>METRDDFMFELSDKPLLPCYNLQVSVSRGPCNWFLFSDVLKRLKLSSRIFQARFPHFEITTMPKAEFYRQVASSQLLTPAERPGGLDDRSPPGSSETVELVRYEPDLLRLLGSEVEFQSCNS[2x];>QGTREQLNLCLERLSSGKDKNKSVLQNKYVRCSVRAEVRHLRRVLCHRLMLNPQHVQLLFDN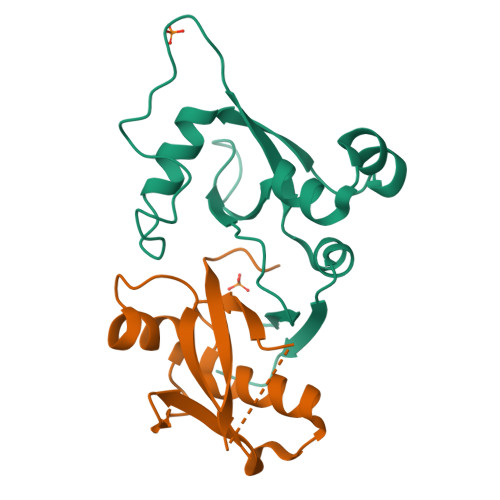EVLPDHMTMKQIWLSRWFGKPSPLLLQYSVK[2x]> MFKKFDEKENVSNCIQLKTSVIKGIK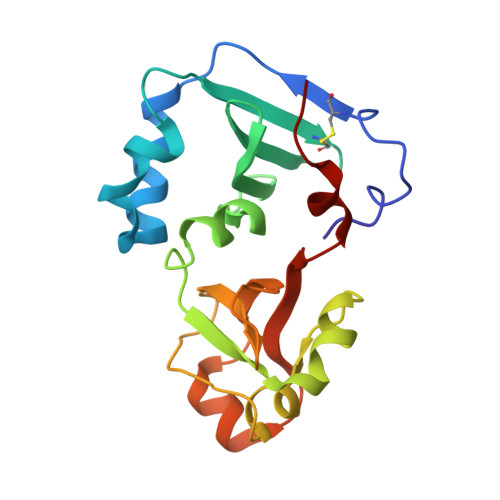NQLIEQFPGIEPWLNQIMPKKDPVKIVRCHEHIEILTVNGELLFFRQREGPFYPTLRLLHKYPFILPHQQVDKGAIKFVLSGANIMCPGLTSPGAKLYPAAVDTIVAIMAEGKQHALCVGVMKMSAEDIEKVNKGIGIENIHYLNDGLWHMKTYK>MSVQLTPHFGNVQAHYDLSDDFFRLFLDPTQTYSCAYFERDDMTLQEAQIAKIDLALGKLNLEPGMTLLDIGCGWGATMRRAIEKYDVNVVGLTLSENQAGHVQKMFDQMDTPRSRRVLLEGWEKFDEPVDRIVSIGAFEHFGHQRYHHFFEVTHRTLPADGKMLLHTIVRPTFKEGREKGLTLTHELVHFTKFILAEIFPGGWLPSIPTVHEYAEKVGFR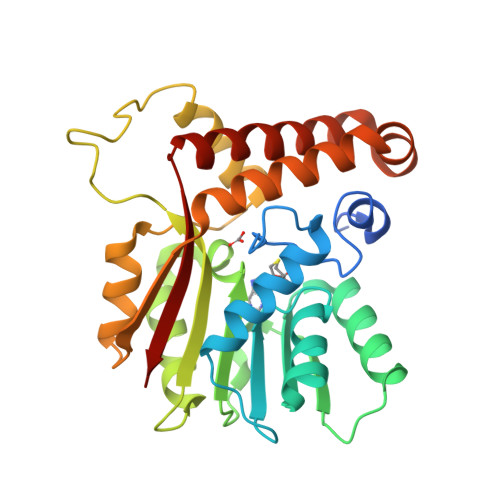VTAVQSLQLHYARTLDMWATALEANKDQAIAIQSQTVYDRYMKYLTGCAKLFRQGYTDVDQFTLEK[2x]4-methoxy-~{N}-phenyl-benzenesulfonamide | C13 H13 N O3 S | 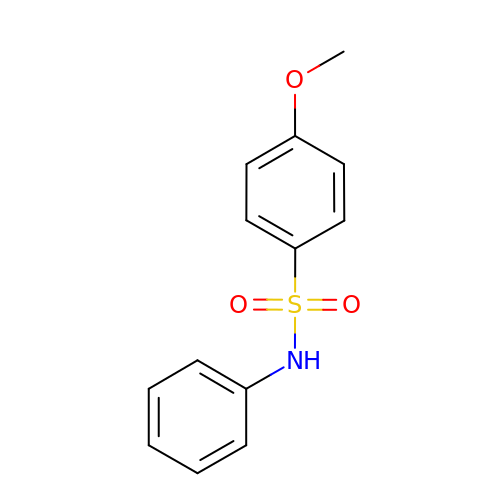GXQBXHZUPPDPLY-UHFFFAOYSA-N Human tyrosyl-DNA phosphodiesterase 1 (TDP1) is a 608 amino acid DNA repair enzyme that processes 3′-DNA end-blocking lesions by hydrolyzing the 3′-phosphate esters. TDP1 is of importance because it can reverse stalled type I topoisomerase (TOP1)-DNA cleavage complexes (TOP1cc′s) by cleaving the phosphodiester bond between the TOP1 Y723 residue and the 3′-phosphate of its DNA substrate (Pommier, 2006; 2009). When acting on TOP1cc′s, the target phosphate ester bond nestles in a well-formed pocket that contains the signature “His-Lys-Asn” (HKN) catalytic residues. As we report herein, we have designed phosphonic acid-containing variants of our previously reported carboxylic acid-containing imidazopyrazine and imidazopyridine inhibitors and we have obtained crystal structures of the catalytic domain of TDP1 (148–608) complexed with a subset of these inhibitors.

In our current work, we obtained X-ray diffraction data from crystals soaked with compounds 3b and 4c at 1.56 Å and 1.58 Å resolution, respectively. In the 1.56 Å data set collected from the TDP1 crystal soaked with 3b, electron density for the arylphosphonic acid headgroup was observed in the active site of both monomers of TDP1 in the asymmetric unit. However, there was no clear electron density observed for the rest of the molecule (imidazopyridine) indicating that this region is disordered likely due to the presence of a rotatable bond between the amino linker and the imidazopyridine moiety. Analysis of the binding mode of the arylphosphonic headgroup demonstrates that each of the oxygen atoms of the phosphonic acid is engaged in binding interactions with the signature HKN catalytic motifs of TDP1. The 01 oxygen atom hydrogen bonds directly to the side chain nitrogen atoms of the K265 and H263 (2.8 Å). The 04 oxygen atom is hydrogen bonded to the side chain nitrogen atom of K495 (3.0 Å) and is engaged in a water-mediated hydrogen bonding network with water 842 (2.8 Å) and the backbone carbonyl oxygen of S514 (2.6 Å). The 03 oxygen atom is hydrogen bonded to the side chain nitrogen atoms of the N283 (2.8 Å) and H493 (2.6 Å). Stabilizing hydrophobic interactions occur between the side chains of Y204 and P461 with the aryl moiety of 3b. When compared to the binding mode of 2b, the phosphonic acid headgroup of 3b superimposes closely with the carboxylate group of 2b (shift of 0.8 Å in distance) and the aryl moieties align closely with a slight rotation of the aryl moiety in 3b. Interactions of the vanadate phosphate mimetic and DNA 3′-phosphate group correspond closely to what we observed with the phosphonic acid in 3b.

>[2x]SGEGQDIWDMLDKGNPFQFYLTRVSGVKPKYNSGALHIKDILSPLFGTLVSSAQFNYCFDVDWLVKQYPPEFRKKPILLVHGDKREAKAHLHAQAKPYENISLCQAKLDIAFGTHHTKMMLLLYEEGLRVVIHTSNLIHADWHQKTQGIWLSPLYPRIADGTHKSGESPTHFKADLISYLMAYNAPSLKEWIDVIHKHDLSETNVYLIGSTPGRFQGSQKDNWGHFRLKKLLKDHASSMPNAESWPVVGQFSSVGSLGADESKWLCSEFKESMLTLGKESKTPGKSSVPLYLIYPSVENVRTSLEGYPAGGSLPYSIQTAEKQNWLHSYFHKWSAETSGRSNAMPHIKTYMRPSPDFSKIAWFLVTSANLSKAAWGALEKNGTQLMIRSYELGVLFLPSAFGLDSFKVKQKFFAGSQEPMATFPVPYDLPPELYGSKDRPWIWNIPYVKAPDTHGNMWVPS> PISPIETVPVKLKPGMDGPKVKQWPLTEEKIKALVEICTEMEKEGKISKIGPENPYNTPVFAIKKKDSTKWRKLVDFRELNKRTQD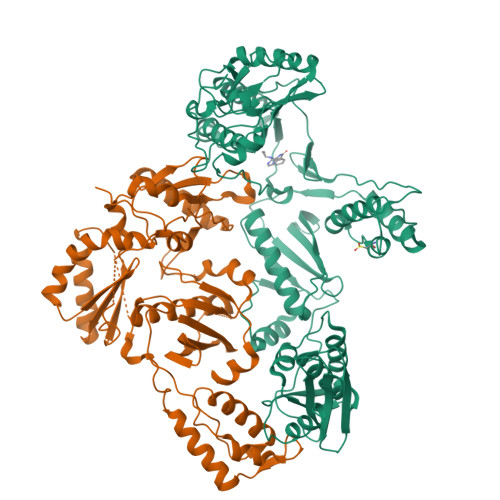FWEVQLGIPHPAGLKKKKSVTILDVGDAYFSVPLDEDFRKYTAFTIPSINNETPGIRYQYNVLPQGWKGSPAIFQSSMTKILEPFRKQNPDIVIYQYMDDLYVGSDLEIGQHRTKIEELRQHLLRWGLTTPDKKHQKEPPFLWMGYELHPDKWTVQPIVLPEKDSWTVNDIQKLVGKLNWASQIYPGIKVRQLCKLLRGTKALTEVIPLTEEAELELAENREILKEPVHGVYYDPSKDLIAEIQKQGQGQWTYQIYQEPFKNLKTGKYARMRGAHTNDVKQLTEAVQKITTESIVIWGKTPKFKLPIQKETWETWWTEYWQATWIPEWEFVNTPPLVKLWYQLEKEPIVGAETFYVDGAANRETKLGKAGYVTNRGRQKVVTLTDTTNQKTELQAIYLALQDSGLEVNIVTDSQYALGIIQAQPDQSESELVNQIIEQLIKKEKVYLAWVPAHKGIGGNEQVDKLVSAGIRKVL;> PISPIETVPVKLKPGMDGPKVKQWPLTEEKIKALVEICTEMEKEGKISKIGPENPYNTPVFAIKKKDSTKWRKLVDFRELNKRTQDFWEVQLGIPHPAGLKKKKSVTILDVGDAYFSVPLDEDFRKYTAFTIPSINNETPGIRYQYNVLPQGWKGSPAIFQSSMTKILEPFRKQNPDIVIYQYMDDLYVGSDLEIGQHRTKIEELRQHLLRWGLTTPDKKHQKEPPFLWMGYELHPDKWTVQPIVLPEKDSWTVNDIQKLVGKLNWASQIYPGIKVRQLCKLLRGTKALTEVIPLTEEAELELAENREILKEPVHGVYYDPSKDLIAEIQKQGQGQWTYQIYQEPFKNLKTGKYARMRGAHTNDVKQLTEAVQKITTESIVIWGKTPKFKLPIQKETWETWWTEYWQATWIPEWEFVNTPPLVKLWYQLEKEPIVGAETF> RGSHMNIKQFDILYIDLNPTRGREKHNVRPCLVINNQMSIDGTNFV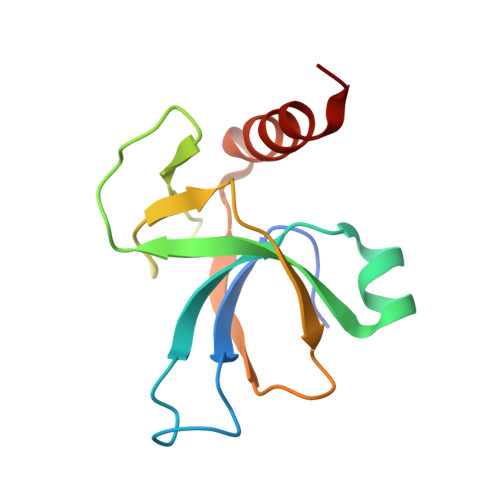WVLPITTRGLRYPTDIQLKTKKGLVSGVIDTVQIRALDLKARQYNYKDELQDNLKNDILKAIKTYLKPTL> HTVELNEMFGQIQSPGYPDSYPSDSEVTWNITVPEFRVQLYFMHFNLESSYLCEYDYVKVETEDQVLATFCGRETTDTEQTPGQEVVLSPGSFMSVTFRSDFSNEERFTGFDAHYMAVDVDECKERED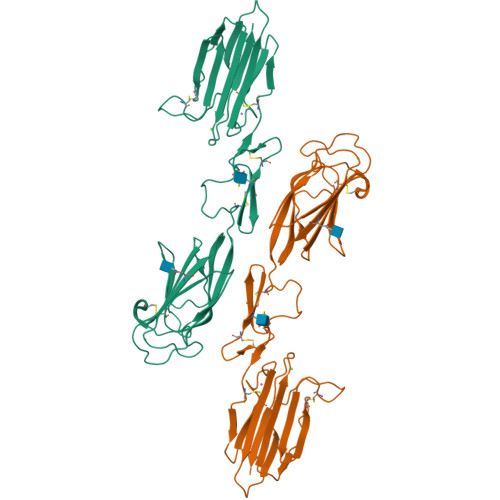EELSCDHYCHNYIGGYYCSCRFGYILHTDNRTCRVECSGNLFTQRTGTITSPDYPNPYPKSSECSYTIDLEEGFMVTLHFEDIFDIEDHPEVPCPYDYIKIKAGSKVWGPFCGEKSPEPISTQSHSIQILFRSDNSGENRGWRLSYRA1-cyclohexyl-3-(2-pyridin-4-ylethyl)urea | C14 H21 N3 O | 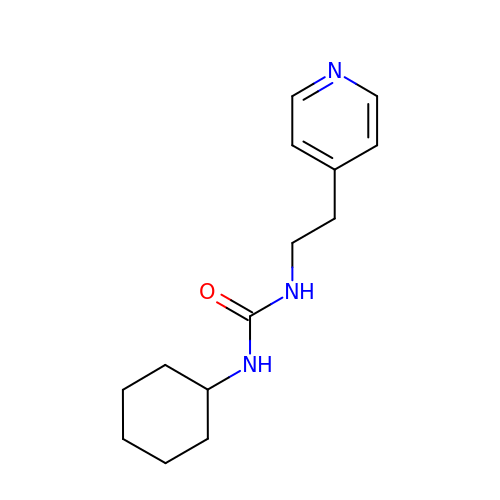XUPGANVQJLTRNJ-UHFFFAOYSA-N>[3x]MFEEINDFETAFKRLLNEVLEFDLQNPLKDVKKVLCIEPHPDDCVIGMGGTIKRLTDRGIEVIYICMTDGYMGTTDENITGHELAQIRRKEEEESAKMLGVKKIYWLNYRDTELPYSREVRKDLVKIIRKEKPDGVFLPDPWLPYEAHPDHRATGFLALDAVAFSPLPNFSNIDLDIGLKPHSVSFIGLYYTSRPNYFVDITDVMDLKLKAIRAHKSQFPDDIWETWEPFLRTVALYYGQKAGVKYAEGFRIMPGLFYHITPFAELI

Deacetylase from the extremophile Pyrococcus chitonophagus has been analyzed by X-ray crystallography, small-angle X-ray scattering, differential scanning calorimetry, isothermal titration calorimetry and NMR to determine its structure, thermodynamics and enzymatic properties. It is a hexameric, zinc-containing metalloenzyme that retains its structural integrity up to temperatures slightly exceeding 100 °C. It removes the acetyl group specifically from the non-reducing end of the sugar substrate. Pch-Dac crystallizes as ‘a dimer of trimers’, with two doughnut-shaped trimers stacked back-to-back along a molecular three-fold axis, with a 8–10 Å channel through the middle of this assembly.

Three crystal forms were analyzed, including monoclinic crystals of the protein-substrate complex (Pch-Dac-lig), having two protein hexamers in the crystal’s asymmetric unit and trigonal crystals of the unliganded protein (Pch-Dac), having half a hexamer in the asymmetric unit, with the other half being related by the crystallographic two-fold axis. In Pch-Dac and Pch-Dac-anom, there was no ligand in the substrate-binding sites and the coordination sphere of Zn2+ consists of the three conserved His-Asp-His residues and a single water molecule that occupies the same position as the carbonyl oxygen of the substrate’s N-acetyl group in the Pch-Dac-lig complex. Thus, with or without the substrate, the Zn2+ cation is coordinated tetrahedrally. Three of its ligands are provided by the protein’s conserved His-Asp-His triad and the fourth, in an unliganded structure, is a single water molecule wedged between two catalytic residues, His259* and Asp42. Two neighboring Pch-Dac hexamers had been extracted from the trigonal crystal lattice and used to improve the curve fitting. The same hexameric assembly is observed regardless of crystal packing and probably represents the biologically relevant oligomeric form of the enzyme.> SSLPQSFLLKSLEQVRKIQGDGAALQEKLCATYKLCHPEELVLLGHSLGIPWAPLSSCPSQALQLAGCLSQLHSGLFLYQGLLQALEGISPELGPTLDTLQLDVADFATTIWQQMEELGMAPALQPTQGAMPAFASAFQRRAGGVLVASHLQSFLEVS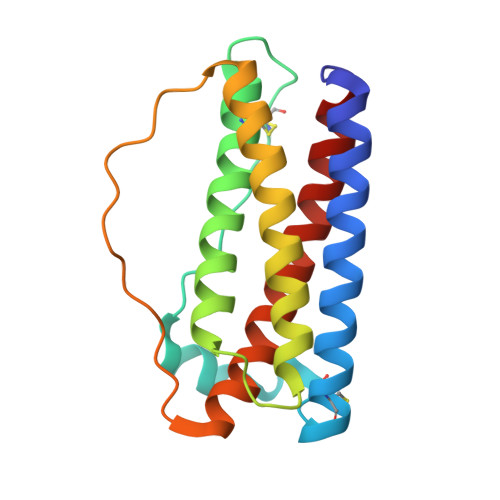YRVLRHLG> MATIAAPGARPRAQAAPGKLVEMNWDPITRIVGSLGIYTKIDFENRRVAECYSTSSIFRGYSIFMKGKDPRDSHFITSRICGICGDNHATCSVYAQNMAYGVKPPPIADWIINLGEAAEYMFDHNIFQDNLVGVDFCEQMVRETNPGVWEKAKTAEAPHAAEHGYRTIADIMTALNPFTGEFYRETLLVS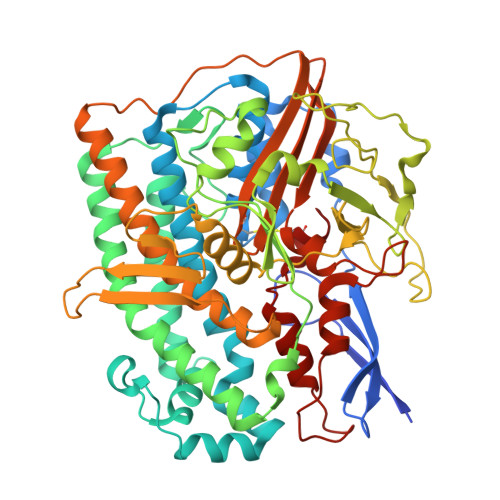RYTREMFCLMEGRHVHPSTLYPGGVGTVPTIQLFTDYITRLMKYVEFMKKVVPLHDDLFDFFYEALPGYEEVGRRRILLGCWGSFQDPNVCDYNYRTMTKWGRGMFVTPGVVVDGELLTTDLVDINLNIRILLGSSFYQDWDHEETSVKNDPLGNAVDRKHPWNQTTLPRPQKRNFGGNYTWVMSPRWLDKRTGDHLALDTGGGPIARLWATALAGLVDIGYIKSTGHSVKIYLPRTALKPEAEFEWKIPMWSNAIERDRARTYFQAYSAAAALYFAEQALAELHAGRTRTFTDFKVPDEAIGCGFHEAVRGVLSHHLVIRDGKIANYHPYPPTPWNASPRDIYGTPGPYEDAVQNTPIFEENGPEKFKGIDIMRAVRSFDPCLPCGVH N-{(1S)-2-({(1S,2R)-1-(3,5-DIFLUOROBENZYL)-3-[(3-ETHYLBENZYL)AMINO]-2-HYDROXYPROPYL}AMINO)-2-OXO-1-[(PENTYLSULFONYL)METHYL]ETHYL}NICOTINAMIDE 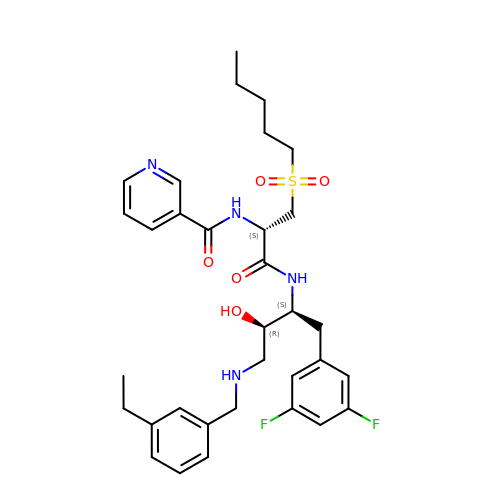| C33 H42 F2 N4 O5 S | IOTPZWJUHSYLHJ-OJDZSJEKSA-N>[6x]MEQRITLKDYAMRFGQTKTAKD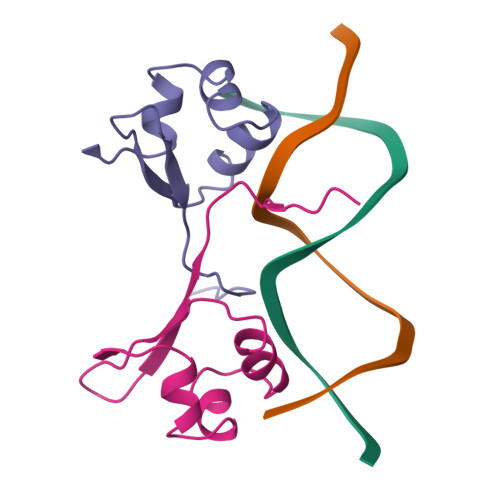LGVYQSAINKAIHAGRKIFLTINADGSVYAEEVKPFPSNKKTTA> SNATDTAEQVIASFRILASDKPYILAEELRRELPPDQAQYCIKRMPAYSGPGSV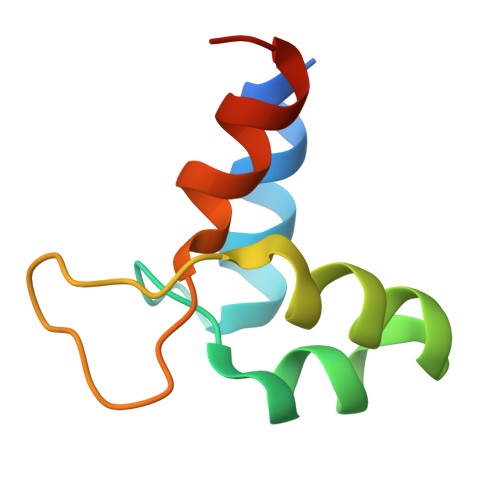PGALDYAAFSSALYGESDL> MPVRRGHVAPQNTFLGTIIRKFEGQNKKFIIANARVQNCAIIYCNDGFCEMTGFSRPDVMQKPCTCDFLHGPETKRHDIAQIAQALLGSEERKVEVTYYHKNGSTFICNTHIIPVKNQEGVAMMFI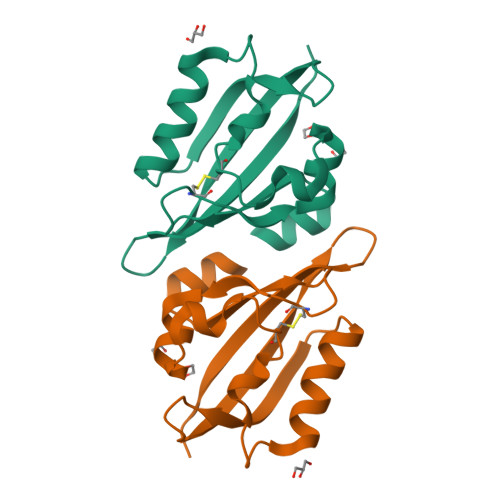INFEYVTDN> MDITRFKEDLKAHLEEKIIPFWQSLKDDEFGGYYGYMDFNLNIDRKAQKGCILNSRILWFFSACYNVLKSEKCKEMAFHAFEFLKNKFWDKEYEGLFWSVSHKGVPVDVTKHVYVQAFGIYGLSEYYEAS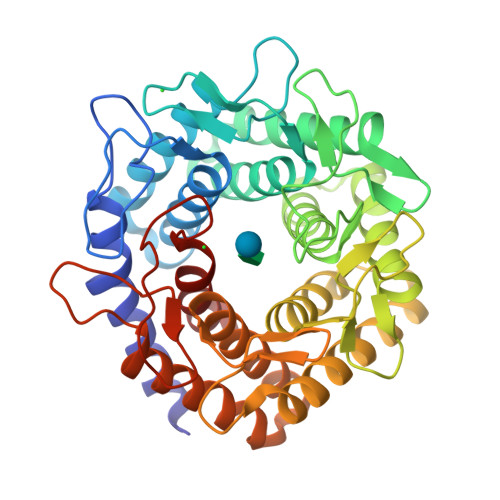GDEEALHMAKRLFEILETKCKRENGYTEQFERNWQEKENRFLSENGVIASKTMNTHLHVLESYTNLYRLLKLDDVYEALEWIVRLFVDKIYKKGTGHFKVFCDDNWNELIKAVSYGHDIEASWLLDQAAKYLKDEKLKEEVEKLALEVAQITLKEAFDGQSLINEMIEDRIDRSKIWWVEAETVVGFFNAYQKTKEEKYLDAAIKTWEFIKEHLVDRRKNSEWLWKVNEDLEAVNMPIVEQWKCPYHNGRMCLEIIKRV>MHHHHHHAASGQPISLMDGKLSFSLPADMTDQSGKLGTQANNMHVYSDPTGQKAVIV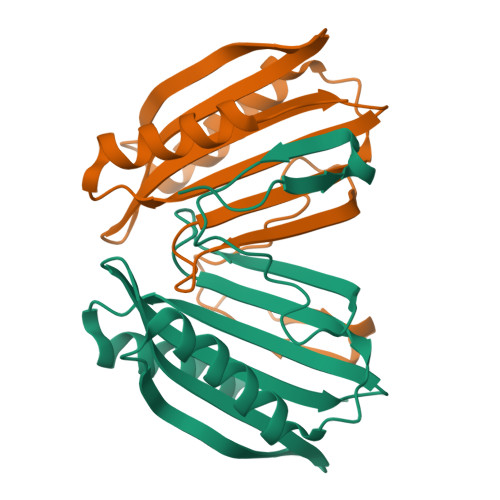IVGDNTDEALPVLANRLLEQQRSRDPQLQVVTNKSIELKGHTLQQLDSIISAKGQTAYSSIVLGKVDNQLLTIQVTLPADNQQKAQTTAENIINTLVIK[2x]> SLFKDDIQLNEHQVAWYSKDWTAVQSAADSFKEKAENEFFEIIGAINNKTKCSIAQKDYSKFMVENALSQFPECMPAVYAMNLIGSGLSDEAHFNYLMAAVPRGKRYGKWAKLVEDSTEVLIIKLLAKRYQVNTNDAINYKSILTKNGKLPLVLKELKGLVTDDFLKEVTKNVKEQKQLKKLALEWGLE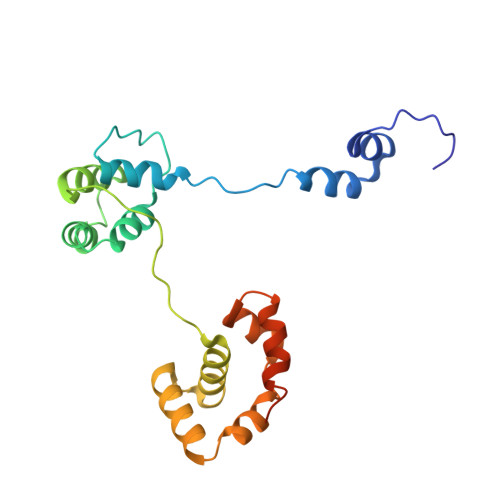HHHHHHHHHH>[2x]GSGMQPDMSLNVIKMKSSDFLESAELDSGGFGKVSLAFHRTQGLMIMKTVYKGPNCIEHNEALLEEAKMMNRLRHSRVVKLLGVIIEEGKYSLVMEYMEKGNLMHVLKAEMSTPLSVKGRIILEIIEGMAYLHGKGVIHKDLKPENIL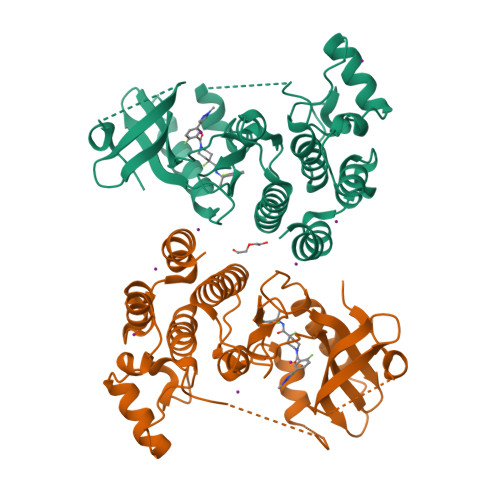VDNDFHIKIADLGLASFKMWSKLNNEEHNELREVDGTAKKNGGTLYYMAPEHLNDVNAKPTEKSDVYSFAVVLWAIFANKEPYENAIAEQQLIMAIKSGNRPDVDDITEYCPREIISLMKLCWEANPEARPTFPGIEEKFRPFYLSQLE>[3x]GAMGSLIRKKAAGLESAATIRTKVFVWGLNDKDQLGGLK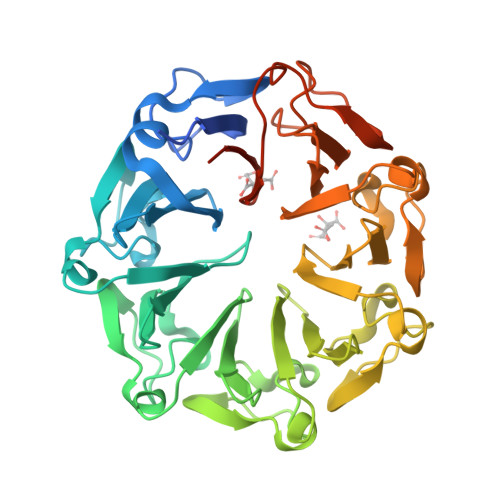GSKIKVPSFSETLSALNVVQVAGGSKSLFAVTVEGKVYACGEATNGRLGLGISSGTVPIPRQITALSSYVVKKVAVHSGGRHATALTVDGKVFSWGEGDDGKLGHFSRMNCDKPRLIEALKTKRIRDIACGSSHSAALTSSGELYTWGLGEYGRLGHGDNTTQLKPKMVKVLLGHRVIQVACGSRDAQTLALTDEGLVFSWGDGDFGKLGRGGSEGCNIPQNIERLNGQGVCQIECGAQFSLALTKSGVVWTWGKGDYFRLGHGSDVHVRKPQVVEGLRGKKIVHVAVGALHCLAVTDSGQVYAWGDNDHGQQGNGTTTVNRKPTLVQGLEGQKITRVACGSSHSVAWTTVDVATPSVHEPVLFQT Like BldD and BldO, BldC acts as a repressor to sustain vegetative growth, and so deletion of bldC causes the premature onset of sporulation. bldC encodes a 68-residue protein that is predicted to contain a winged helix-turn-helix (wHTH) motif, suggesting it may be involved in DNA binding. While BldC appears to contain a MerR-like wHTH, it is to date, the only known MerR-like protein that consists entirely of a wHTH with no obvious effector or oligomerization domain. Using a battery of structural, biochemical, and in vivo approaches, we show here that BldC functions as a pleotropic regulator of Streptomyces development by employing a unique mode of DNA binding for a transcription factor that involves asymmetric head-to-tail oligomerization on DNA direct repeats of varying number with concomitant distortion of the DNA.

To deduce the molecular basis for this extended binding we next determined the structure of BldC in complex with an 18mer smeA-ssfA DNA fragment that contained the first two repeats of the smeA-ssfA BldC binding site, 5′-GCAATTCGGTCGAATTTC-3′. The DNA was constructed to generate pseudo-continuous packing of the DNA, which was indeed generated in the crystals. The structure was solved by molecular replacement (MR) and refined to Rwork/Rfree values of 20.9%/27.8% to 3.09 Å resolution. The structure reveals a striking extended protein-nucleic acid filament with multiple BldC subunits arranged in the same head-tail manner as observed in the BldC-whiI opt structure. The asymmetric BldC dimer contacts and DNA docking mode in this structure are identical to those observed in the BldC-whiI opt structure. Indeed, due to the continuous stacking of the DNA, it was possible that the 9 bp sites bound by each BldC subunit are statistically disordered (half of the time containing one 9 bp sequence and the other half, the other 9 bp sequence). To address the possibility that the DNA may be statistically disordered, X-ray intensity data were collected on a crystal grown with DNA containing a thymine to 5-iododeoxyuracil substitution (5′-GTAAXTCGGTCGAATTTC-3′, where X is 5-iododeoxyuracil). An electron density difference map revealed no strong electron density peaks for the iodine indicating that the DNA is statistically disordered. While the DNA contacts in this structure are statistically disordered, the structure reveals how multiple BldC subunits can bind a promoter site with multiple cognate repeats to create an extended protein superstructure. This superstructure results in a continuous electropositive patch that tracks along the length of the DNA. The binding of multiple BldC subunits along the DNA also leads to severe DNA distortion and shortening: the BldC subunits reduce the length of the DNA by a third when compared to canonical B-DNA.

>GSHMTARTPDAEPLLTPAEVATMFRVDPKTVTRWAKAGKLTSIRTLGGHRRYREAEVRALLAGIPQQRSEA[11x]> MKKEVRKVRIALASPEKIRSWSYGEVEKPETINYRTLKPERDGLFDERIFGPIKDYECACGKYKRQRFEGKVCERCGVEVTKSIVRRYRMGHIELATPAAHIWFVKDVPSKIGTLLDLSATELEQVLYFSKYIVLDPKGAILNGVPVEKRQLLTDEEYRELRYGKQETYPLPPGVDALVKDGEEVVKGQELAPGVVSRLDGVALY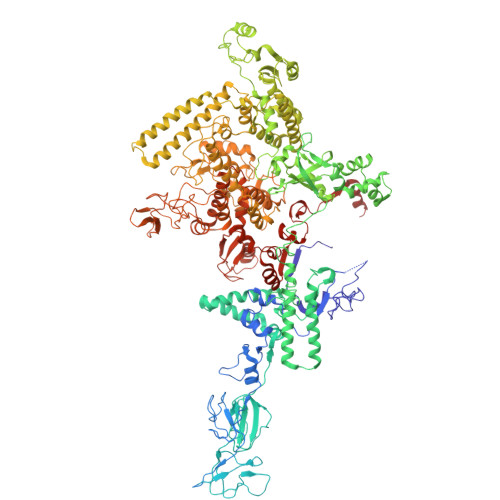RFPRRVRVEYVKKERAGLRLPLAAWVEKEAYKPGEILAELPEPYLFRAEEEGVVELKELEEGAFLVLRREDEPVATYFLPVGMTPLVVHGEIVEKGQPLAEAKGLLRMPRQVRAAQVEAEEEGETVYLTLFLEWTEPKDYRVQPHMNVVVPEGARVEAGDKIVAAIDPEEEVIAEAEGVVHLHEPASILVVKARVYPFEDDVEVSTGDRVAPGDVLADGGKVKSDVYGRVEVDLVRNVVRVVESYDIDARMGAEAIQQLLKELDLEALEKELLEEMKHPSRARRAKARKRLEVVRAFLDSGNRPEWMILEAVPVLPPDLRPMVQVDGGRFATSDLNDLYRRLINRNNRLKKLLAQGAPEIIIRNEKRMLQEAVDALLDNGRRGAPVTNPGSDRPLRSLTDILSGKQGRFRQNLLGKRVDYSGRSVIVVGPQLKLHQCGLPKRMALELFKPFLLKKMEEKGIAPNVKAARRMLERQRDIKDEVWDALEEVIHGKVVLLNRAPTLHRLGIQAFQPVLVEGQSIQLHPLVCEAFNADFDGDQMAVHVPLSSFAQAEARIQMLSAHNLLSPASGEPLAKPSRDIILGLYYITQVRKEKKGAGLEFATPEEALAAHERGEVALNAPIKVAGRETSVGRLKYVFANPDEALLAVAHGIVDLQDVVTVRYMGKRLETSPGRILFARIVAEAVEDEKVAWELIQLDVPQEKNSLKDLVYQAFLRLGMEKTARLLDALKYYGFTFSTTSGITIGIDDAVIPEEKKQYLEEADRKLLQIEQAYEMGFLTDRERYDQILQLWTETTEKVTQAVFKNFEENYPFNPLYVMAQSGARGNPQQIRQLCGLRGLMQKPSGETFEVPVRSSFREGLTVLEYFISSHGARKGGADTALRTADSGYLTRKLVDVTHEIVVREADCGTTNYISVPLFQPDEVTRSLRLRKRADIEAGLYGRVLAREVEVLGVRLEEGRYLSMDDVHLLIKAAEAGEIQEVPVRSPLTCQTRYGVCQKCYGYDLSMARPVSIGEAVGIVAAQSIGEPGTQLTMRTFHTGGVAGAADITQGLPRVIELFEARRPKAKAVISEIDGVVRIEETEEKLSVFVESEGFSKEYKLPKEARLLVKDGDYVEAGQPLTRGAIDPHQLLEAKGPEAVERYLVEEIQKVYRAQGVKLHDKHIEIVVRQMMKYVEVTDPGDSRLLEGQVLEKWDVEALNERLIAEGKTPVAWKPLLMGVTKSALSTKSWLSAASFQNTTHVLTEAAIAGKKDELIGLKENVILGRLIPAGTGSDFVRFTQVVDQKTLKAIEEARKEAVEAKERPAARRGVKREQPGKQA> APAVADKADNAFMMICTALVLFMTIPGIALFYGGLIRGKNVLSMLTQVTVTFALVCILWVVYGYSLAFGEGNNFFGNINWLMLKNIELTAVMGSIYQYIHVAFQGSFACITVGLIVGALAERIRFSAVLIFVVVWLTLSYIPIAHMVWGGGLLASHGALDFAGGTVVAINAAIAGLVGAYLIGKRVGFGKEAFKPHNLPMVFTGTAILYIGWFGFNAGSAGTANEIAALAFVNTVVATAAAILGWIFGEWALRGKPSL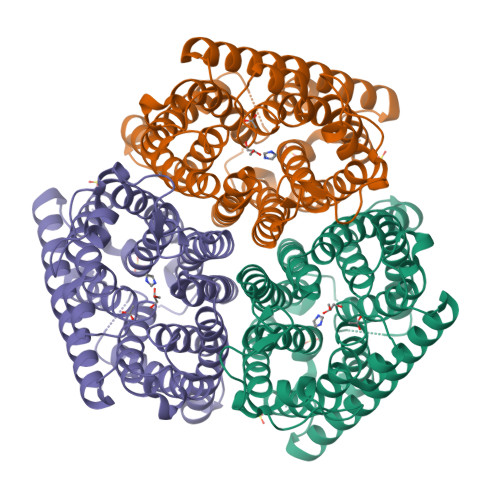LGACSGAIAGLVGVTPACGYIGVGGALIIGVVAGLAGLWGVTMLKRLLRVDDPCDVFGVAGVCGIVGCIMTGIFAASSLGGVGFAEGVTMGHQLLVQLESIAITIVWSGVVAFIGYKLADLTVGLRVPEEQEREGLDVNSHGENAYNADQAQQPAQADLEHHHHHH> MKPEIEQELSHTLLTELLAYQFASPVRWIETQDVFLKQHNTERIIEIGPSPTLAGMANRTIKAKYESYDAALSLQRQVLCYSKDAKEIYYKPDPADLAPKETPKQEESTPSAPAAATPTPAAAAAPTPAPAPASAGPVESIPDEPVKANLLIHVLVAQKLKKPLDAVPMTKAIKDLVNGKSTVQNEILGDLGKEFGSTPEKPEDTPLEELAEQFQDSFSGQLGKTSTSLIGRLMSSKMPGGFSITTARKYLESRFGLGAGRQDSVLLMALTNEPANRLGSEADAKTFFDGIAQKYASSAGISLSSGAGSGAGAANSGGAVVDSAALDALTAENKKLAKQQLEVLARYLQVDLNKGSAKSFIKEKEASAVLQKELDLWEAEHGEFYAKGIQPTFSALKSRTYDSYWNWARQDVLSMYFDIIFGKLTSVDRETINQCIQIMNRANPTLIKFMQYHIDHCPEYKGETYKLAKRLGQQLIDNCKQVLTEDPVYKDVSRITGPKTKVSAKGNIEYEETQKDSVRKFEQYVYEMAQGGAMTKVSQPTIQEDLARVYKAISKQASKDSKLELQRVYEDLLKVVESSKEIETEQLTKDILQAATVPTTPTEEVDDPCTPSSDDEIASLPDKTSIIQPVSSTIPSQTIPFLHIQKKTKDGWEYNKKLSSLYLDGLESAAINGLTFKDKYVLVTGAGAGSIGAEILQGLISGGAKVIVTTSRFSKKVTEYYQNMYARYGAAGSTLIVVPFNQGSKQDVDALVQYIYDEPKKGGLGWDLDAIIPFAAIPENGNGLDNIDSKSEFAHRIMLTNLLRLLGAVKSKKTTDTRPAQCILPLSPNHGTFGFDGLYSESKISLETLFNRWYSEDWGSKLTVCGAVIGWTRGTGLMSANNIIAEGIEKLGVRTFSQKEMAFNILGLLTPEIVQLCQEEPVMADLNGGLQFIDNLKDFTSKLRTDLLETADIRRAVSIESAIEQKVVNGDNVDANYSKVMVEPRANMKFDFPTLKSYDEIKQIAPELEGMLDLENVVVVTGFAEVGPWGNSRTRWEMEAYGEFSLEGAIEMAWIMGFIKYHNGNLKGKPYSGWVDAKTQTPIDEKDIKSKYEEEILEHSGIRLIEPELFNGYDPKKKQMIQEVVVQHDLEPFECSKETAEQYKHEHGEKCEIFEIEESGEYTVRILKGATLYVPKALRFDRLVAGQIPTGWDARTYGIPEDTISQVDPITLYVLVATVEALLSAGITDPYEFYKYVHVSEVGNCSGSGMGGVSALRGMFKDRYADKPVQNDILQESFINTMSAWVNMLLLSSSGPIKTPVGACATAVESVDIGIETILSGKAKVVLVGGYDDFQEEGSYEFANMNATSNSIEEFKHGRTPKEMSRPTTTTRNGFMEAQGSGIQVIMTADLALKMGVPIHAVLAMTATATDKIGRSVPAPGKGILTTAREHHGNLKYPSPLLNIEYRKRQLNKRLEQIKSWEETELSYLQEEAELAKEEFGDEFSMHEFLKERTEEVYRESKRQVSDAKKQWGNSFYKSDPRIAPLRGALAAFNLTIDDIGVASFHGTSTVANDKNESATINNMMKHLGRSEGNPVFGVFQKYLTGHPKGAAGAWMLNGAIQILESGLVPGNRNADNVDKLLEQYEYVLYPSRSIQTDGIKAVSVTSFGFGQKGAQAVVVHPDYLFAVLDRSTYEEYATKVSARNKKTYRYMHNAITRNTMFVAKDKAPYSDELEQPVYLDPLARVEENKKKLVFSDKTIQSSQSYVGEVAQKTAKALSTLNKSSKGVGVDVELLSAINIDNETFIERNFTGNEVEYCLNTAHPQASFTGTWSAKEAVFKALGVESKGAGASLIDIEITRDVNGAPKVILHGEAKKAAAKAGVKNVNISISHDDFQATAVALSEF;> MSTHRPFQLTHGSIEHTLLVPNDLFFNYSQLKDEFIKTLPEPTEGFAGDDEPSSPAELYGKFIGFISNAQFPQIVELSLKDFESRFLDNNNDNIHSFAVKLLDDETYPTTIAKVKENIVKNYYKAVKSINKVESNLLYHCKHDAKLVAIFGGQGNTDDYFEELRELYTLYQGLIEDLLVSIAEKLNQLHPSFDKIYTQGLNILSWLKHPETTPDQDYLLSVPVSCPVICVIQLCHYTITCKVLGLTPGEFRNSLKWSTGHSQGLVTAVTIAASDSWDSFLKNSLTAVSLLLFIGSRCLSTYPRTSLPPTMLQDSLDNGEGRPSPMLSVRDLSIKQVEKFIEQTNSHLPREKHIAISLINGARNLVLSGPPESLYGFNLNLRNQKAPMGLDQSRVPFSERKLKCSNRFLPIFAPFHSHLLADATELILDDVKEHGLSFEGLKIPVYDTFDGSDFQALKEPIIDRVVKLITELPVHWEEATNHKATHILDFGPGGVSGLGVLTHRNKEGTGARIILAGTLDSNPIDDEYGFKHEIFQTSADKAIKWAPDWLKELRPTLVKNSEGKIYVKTKFSQLLGRAPLMVAGMTPTTVNTDIVSASLNAGYHIELAGGGYFSPVMMTRAIDDIVSRIKPGYGLGINLIYVNPFMLQWGIPLIKDLREKGYPIQSLTIGAGVPSIEVATEYIEDLGLTHLGLKPGSVDAISQVIAIAKAHPTFPIVLQWTGGRGGGHHSFEDFHQPIIQMYSKIRRCSNIVLVAGSGFGSDEDTYPYLSGYWSEKFNYPPMPFDGVLFGSRVMTSKESHTSLAAKKLIVECKGVPDQQWEQTYKKPTGGIITVRSEMGEPIHKIATRGVMFWKELDDTIFNLPKNKLLDALNKKRDHIIKKLNNDFQKPWFGKNANGVCDLQEMTYKEVANRLVELMYVKKSHRWIDVSLRNMYGDFLRRVEERFTSSAGTVSLLQNFNQLNEPEQFTADFFEKFPQAGKQLISEEDCDYFLMLAARPGQKPVPFVPVLDERFEFFFKKDSLWQSEDLESVVDEDVQRTCILHGPVASQYTSKVDEPIGDILNSIHEGHIARLIKEEYAGDESKIPVVEYFGGKKPASVSATSVNIIDGNQVVYEIDSELPNKQEWLDLLAGTELNWLQAFISTDRIVQGSKHVSNPLHDILTPAKHSKVTIDKKTKKLTAFENIKGDLLPVVEIELVKPNTIQLSLIEHRTADTNPVALPFLYKYNPADGFAPILEIMEDRNERIKEFYWKLWFGSSVPYSNDINVEKAILGDEITISSQTISEFTHAIGNKCDAFVDRPGKATLAPMDFAIVIGWKAIIKAIFPKSVDGDLLKLVHLSNGYKMITGAAPLKKGDVVSTKAEIKAVLNQPSGKLVEVVGTIYREGKPVMEVTSQFLYRGEYNDYCNTFQKVTETPVQVAFKSAKDLAVLRSKEWFHLEKDVQFDVLTFRCESTYKFKSANVYSSIKTTGQVLLELPTKEVIQVGSVDYEAGTSYGNPVTDYLSRNGKTIEESVIFENAIPLSSGEELTSKAPGTNEPYAIVSGDYNPIHVSRVFAAYAKLPGTITHGMYSSASIRALVEEWAANNVAARVRAFKCDFVGMVLPNDTLQTTMEHVGMINGRKIIKVETRNVETELPVLIGEAEIEQPTTTYVFTGQGSQEQGMGMELYNSSEVAREVWDKADRHFVNNYGFSILDIVQNNPNELTIHFGGAKGRAIRDNYIGMMFETIGEDGALKSEKIFKDIDETTTSYTFVSPTGLLSATQFTQPALTLMEKAAYEDIKSKGLIPSDIMFAGHSLGEYSALSSLANVMPIESLVDVVFYRGMTMQVAVPRDELGRSNYGMVAVNPSRVSATFDDSALRFVVDEVANKTKWLLEIVNYNVENQQYVAAGDLRALDTLTNVLNVLKINKIDIVKLQEQMSIEKVKEHLYEIVDEVAAKSLAKPQPIDLERGFAVIPLKGISVPFHSSYLMSGVKPFQRFLCKKIPKSSVKPQDLIGKYIPNLTAKPFELTKEYFQSVYDLTKSEKIKSILDNWEQYE

Type I fungal FAS forms a barrel-shaped complex composed of two reaction chambers. Six β-chains form the walls of the barrel while a central wheel, made by the six α-chains, bisects the barrel into two chemically identical reaction chambers. Therefore, each chamber has three complete sets of catalytic domains including three acyl-carrier protein (ACP) domains. Substrates are shuttled between the static reaction centers by the mobile ACP domain flexibly tethered at its N and C termini.

In the Apo state, ACP density is strongest in proximity of the KS domain in S. cerevisiae FAS and allows for a complete tracing of its backbone atoms in the high resolution cryoEM map. In the Apo state of C. albicans (62 and 69% identity for β- and α-chains, relative to their respective S. cerevisiae chains), the ACP density is strongest in proximity of the ER domain, similarly allowing for complete tracing of the backbone atoms of this mobile domain at an alternate location. However, the negative surface charge on KS domain is weakened in C. albicans due to alteration of some of the acidic residues that form the interface with the structural lobe of ACP. Weaker charge complementarity can partly explain why in this pathogenic fungal species, ACP is not primarily localized at the KS in the Apo state. Interestingly, unlike the KS-binding site where both canonical and structural lobes of ACP contribute to the surface area of the binding interface, the interface of ACP at the ER mainly involves the canonical lobe. This observation can explain the worse local resolution seen for the ACP of C. albicans localized at the ER compared to that in S. cerevisiae at the KS domain in the Apo states. In the Apo state of C. albicans FAS, the second strongest density is in proximity of the KS domain that is only observable at lower resolution and threshold of the AAI cryoEM density map. In both FASs in the Apo state, the structural lobe of ACP has stronger and better resolved densities compared to the canonical lobe in the KS-binding site, as observed in the high-resolution refined maps, suggesting a more stable interaction between the former and the KS-domain in the absence of substrates. Examining the ER active site in C. albicans Apo state where ACP is partially bound, we can clearly see the density of the phosphopantetheine arm until the quaternary carbon atom of the moiety. Interestingly, the catalytic histidine can be modeled with two side chain orientations, one facing FMN and the other facing the phosphate group of the phosphopantetheine arm. Based on these structures, the catalytic histidine in the ER domain of type I fungal FAS may sample alternative conformations to form a proton transfer bridge between FMN and the enoyl functional group of the elongating fatty acid chain when ACP is bound.>CUGGGCGG[2x];>CCGCCUGG[2x]

We have obtained crystals of a racemic compound consisting of l- and d-RNA duplexes in which the enantiomers pack in the crystal lattice in an asymmetric manner and show differences in their structures, crystal contacts and interactions with the solvent. The crystals of d- and l-RNA duplexes (CUGGGCGG)-(CCGCCUGG) belong to space group P1 with the unit cell parameters a = 21.1 Å, b = 26.7 Å, c = 39.1 Å, α = 105.9°, β = 97.0°, and γ = 91.6°. The unit cell contains one d-RNA duplex and one l-RNA duplex stacking head-to-tail, arranged in the crystal lattice into parallel semi-infinite columns. The d-duplexes have the helical parameters characteristic of A-RNA, while the l-duplexes take values appropriately inverted for the other enantiomer.

The absolute configuration of the structure was determined for each analyzed crystal using the anomalous dispersion of X-rays from the Zn2+ ions. Of the nine crystals that gave diffraction data containing statistically significant anomalous signals, seven crystals had the K:L RNA duplex in the d-configuration, and the M:N duplex was in the l-configuration. The remaining two crystals had the inverted configuration l-(K:L)/d-(M:N). Of the eight crystals that gave no statistically significant anomalous signal but gave anomalous peaks at the Zn2+ ions, four crystals were d-(K:L)/l-(M:N), and four were l-(K:L)/d-(M:N). The ratio of the d-(K:L)/l-(M:N) to l-(K:L)/d-(M:N) crystal structures, of 7 to 2 for the best data sets and 11 to 6 overall, does not indicate a clear bias. The intermolecular crystal contacts of the two enantiomers are also different. When the two duplexes (K:L and M:N) are compared, chain K is more exposed to the solvent than its corresponding enantiomer, chain M, which makes more extensive contacts with neighboring RNA molecules. The percentage ratio of the solvent-exposed surface area to the intermolecular crystal contact area is 72/28 for chain K and 57/43 for chain M. The situation is reversed for the other strands of the two duplexes: the ratios of the solvent-exposed intermolecular contact areas are 55/45 for chain L and 71/29 for chain N. Asymmetry between the RNA enantiomers is also observed in their interactions with the Zn2+ ions. In the presented structure, one enantiomer interacts with three zinc cations, while the other interacts with four zinc cations.> MEPEEERIRYSQRLRGTMRRRYEDDGISDDEIEGKRTFDLEEKLHTNKYNANFVTFMEGKDFNVEYIQRGGLRDPLIFKNSDGLGIKMPDPDFTVNDVKMCVGSRRMVDVMDVNTQKGIEMTMAQWTRYYETPEEEREKLYNVISLEFSHTRLENMVQRPSTVDFIDWVDNMWPRHLKESQTESTNAILEMQYPKVQKYCLMSVRGCYTDFHVDFGGTSVWYHIHQGGKVFWLIPPTAHNLELYENWL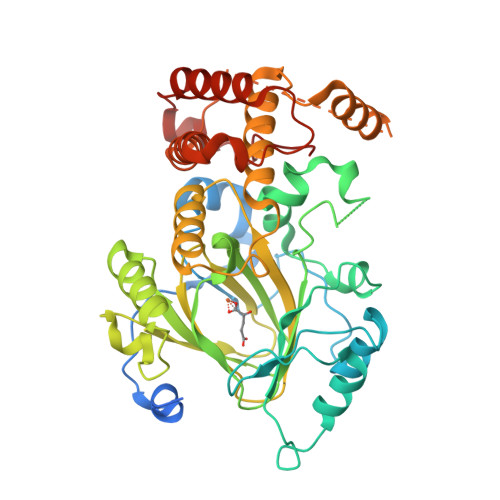LSGSQGDIFLGDRVSDCQRIELKQGYTFVIPSGWIHAVYTPTDTLVFGGNFLHSFNIPMQLKIYNIEDRTRVPNKFRYPFYYEMCWYVLERYVYCITNRSHLTKEFQKESLSMDLELNGLESGNGDEEAVDREPRQVHLTHFELEGLRCLVDKLESLPLHKKCVPTGIEDEDALIADVKILLEELANSDPKLALTGVPIVQWP> DLKKNEDLKQMLESNKDSAKLDAMKRIVGMIAKGKNASELFPAVVKNVASKNIEIKKLVYVYLVRYAEEQQDLALLSISTFQRALKDPNQLIRASALRVLSSIRVPIIVPIMMLAIKEASADLSPYVRKNAAHAIQKLYSLDPEQKEMLIEVIEKLLKDKSTLVAGSVVMAFEEVCPDRIDLIHKNYRKLCNLLVDVEEWGQVVIIHMLTRYARTQFVSPWDPDHRLLIRNTKPLLQSRNAAVVMAVAQLYWHISPKSEAGIISKSLVRLLRSNREVQYIVLQNIATMSIQRKGMFEPYLKSFYVRSTDPTMIKTLKLEILTNLANEANISTLLREFQTYVKSQDKQFAAATIQTIGRCATNILEVTDTCLNGLVCLLSNRDEIVVAESVVVIKKLLQMQPAQHGEIIKHMAKLLDSITVPVARASILWLIGENCERVPKIAPDVLRKMAKSFTSEDDLVKLQILNLGAKLYLTNSKQTKLLTQYILNLGKYDQNYDIRDRTRFIRQLIVPNVKSGALSKYAKKIFLAQKPAPLLESPFKDR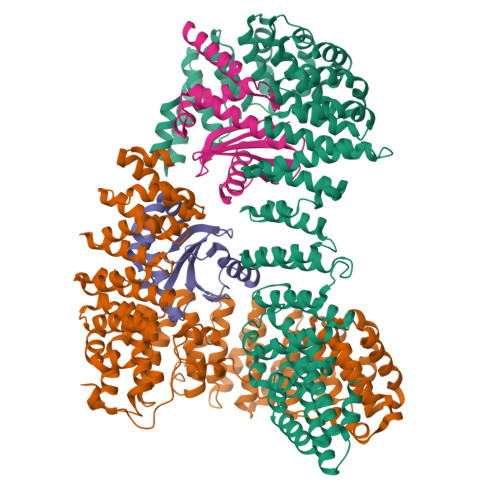DHFQLGTLSHTLNIKATGYLELSNWPEVAPDPSVRN;> LQDLVRGIRNHKEDEAKYISQCIDEIKQELKQDNIAVKANAVCKLTYLQMLGYDISWAAFNIIEVMSASKFTFKRIGYLAASQSFHEGTDVIMLTTNQIRKDLSSPSQYDTGVALTGLSCFVTPDLARDLANDIMTLMSHTKPYIRKKAVLIMYKVFLKYPESLRPAFPRLKEKLEDPDPGVQSAAVNVICELARRNPKNYLSLAPLFFKLMTSSTNNWVLIKIIKLFGALTPLEPRLGKKLIEPLTNLIHSTSAMSLLYECVNTVIAVLISLSSGMPNHSASIQLCVQKLRILIEDSDQNLKYLGLLAMSKILKTHPKSVQSHKDLILQCLDDKDESIRLRALDLLYGMVSKKNLMEIVKKLMTHVDKAEGTTYRDELLTKIIDICSQSNYQYITNFEWYISILVELTRLEGTRHGHLIAAQMLDVAIRVKAIRKFAVSQMSALLDSAHLLASSTQRNGICEVLYAAAWICGEFSEHLQEPHHTLEAMLRPRVTTLPGHIQAVYVQNVVKLYASILQQKEQAGEAEGAQAVTQLMVDRLPQFVQSADLEVQERASCILQLVKHIQKLQAKDVPVAEEVSALFAGELN;> MIHSLFLINCSGDIFLEKHWKSVVSQSVCDYFFEAQEKAADVENVPPVISTPHHYLISIYRDKLFFVSVIQTEVPPLFVIEFLHRVADTFQDYFGECSEAAIKDNVVIVYELLEEMLDNGFPLA;> MIKAILIFNNHGKPRLSKFYQPYSEDTQQQIIRETFHLVSKRDENVCNFLEGGLLIGGSDNKLIYRHYATLYFVFCVDSSESELGILDLIQVFVETLDKCFENVCELDLIFHVDKVHNILAEMVMGGMVLETNMNEIVTQIDAQNKLEKSE(1S)-2,2-difluoro-1-[1-(pentan-3-yl)-1H-pyrazol-4-yl]ethan-1-ol 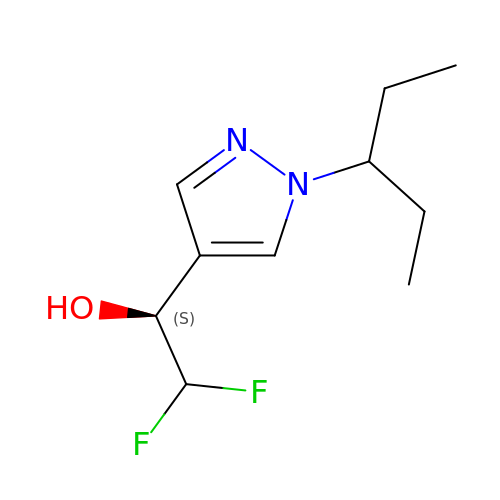| C10 H16 F2 N2 O | LKTXIVWHOJXFEW-VIFPVBQESA-N>MAEAFTREDYVFMAQLNENAERYDEMVETMRKISGMEGELSDKERNLLSVAYKNVIGPRRAAWRIVSSIEAKEKG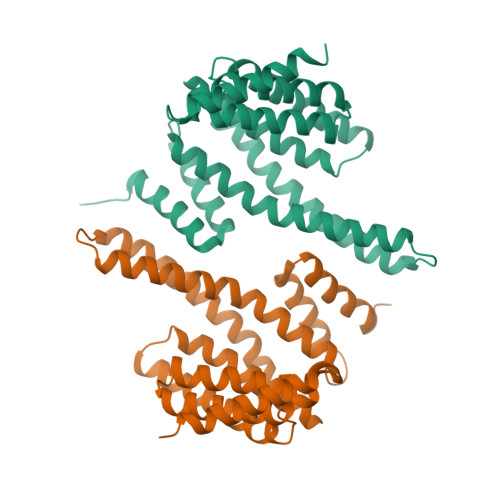RQKPNAKRIEQIRVYRQKIEKELSDICNDILKLLQEQFVPRSTNADAKVFYYKMQGDYYRYLAEYSSGEDKEKIAGSALNAYNSAFEISQQLPPTHPIRLGLALNFSVFYYEILASPDRACELARKAFDAAITDLDKLTEESYKDSTLIMQLLRDNLNLWVTDSAGDDNAEGGGGGGGGGG[4x]>MDATALERDAVQFARLAVQRDHEGRYSEAVFYYKEAAQALIYAEMAGSSLENIQEKITEYLERVQALHSAVQSKSADPLKSKHQLDLERAHFLVTQAFDEDEKENVEDAIELYTEAVDLCLKTSYETADKVLQNKLKQLARQALDRAEALSEPLTKPVGKISSTS[2x];>NFVLPELP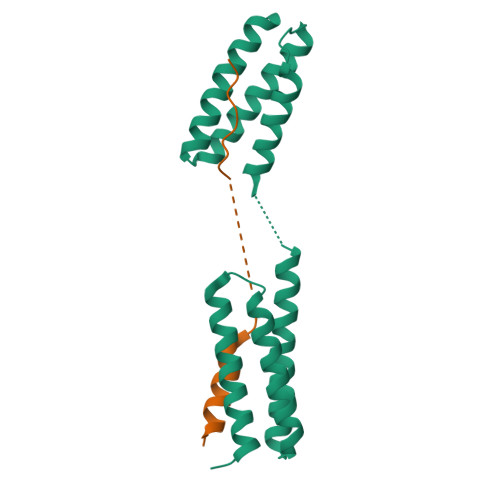SVPDTLPTASAGASTSASEDIDFDDLSRRFEELKKKT[2x]>MNINEPSGEAANIISQAADSHAMKYYNAADWQAEDNALPSLAELRDLVINQQKSVLFDFSQNSDADGQAEMQAQFRKTYGVGFANQFIFITEHKGELLFTPFEHSEEVDPKLLEAPLTTRSGLKSTAPTNSETSTLPHVAFYISVNRPISDEECTFDNSWLWKDEKGSRPFCKDANISLIYRVNLERSLQYGIVGSATPNAKIVRISLDDDSSGAGIHLNDQLSYRRFGASYTTLDAYFREWSTDAIAQDYRFVFKTSNNKAEILETFPIDNLNVKYEKRKQSGFELGVTGGAEVSEDGPKAKLEARASITQSRWLTYNTQDYRVERNAKNAQTVSFTWNRQEYATAESLLNRSTDALWVDTYPVDVNRISPLSYASFVPKMDVIYKASDTETGSTDFIIDSSVNIRPIYNGAYKHYYVVGAHQSYHGFENSPRRRITKSASFTVDWDHPVFTGGRPVNLQLASFNNRCVQVDAQSRLTANTCDDQQSAQSFIYDQLGRYVSASNTELCLDGAALDVLQTCNQNLTQRWEWRKNTDELTNVYSGESLGHDKQTGELGLYASSNDAVSLRTITAYTNVFNVQKSSPILGYTQGKMNQQSVGQNYRLYVREGSAIDALGTASDLLVGGNGGSLTSVDLSGVKSITATSGDFQYGGQQLVALTFTYQDGRQQMVGSKAHVTNAHEDRFDLPDAAKITQLNIWADDWLVKGVQFDLNLEHHHHHH[7x]

Vibrio α-hemolysins (αHLs) are β-pore-forming toxins secreted by Vibrio pathogens, crucial for the facilitation of bacterial infections through host cell lysis. These toxins are produced as inactive precursors, requiring proteolytic maturation and membrane association for activation within host tissues. Here, we investigate Vibrio campbellii αHL (VcαHL), and establish that its hemolytic activity is significantly stimulated by calcium ions, with an EC50 that aligns with physiological calcium concentrations. Using X-ray crystallography and cryo-electron microscopy, we decipher both the immature and assembled structures of VcαHL and elucidate the conformational changes corresponding to toxin assembly.

The VcαHL was assembled on liposomal membranes and solubilized using styrene-maleic acid (SMA), yielding SMA lipid particles (SMALPs) containing assembled VcαHL. Cryo-micrographs of VcαHL in SMALPs were acquired and analyzed for single-particle 3D reconstitution, resulting in a density map of 2.06 Å resolution. The map revealed a heptameric complex exhibiting C7 symmetry, featuring a β-barrel transmembrane pore channel. In contrast, the β-prism lectin domain was not visualized in the map due to its flexible position in the complex, as indicated by the fuzzy cloud observed in 2D classification images. When compared to pro-VcαHL, the protomer of assembled VcαHL displays several conformational changes post pore formation, in addition to the substantial relocation of pre-stem loops. These include a slight clockwise rotation of the β-trefoil lectin domain when observed from the extracellular view and a minor displacement of the cradle loop, which seems to facilitate interaction with the adjacent protomer and release of the pre-stem loop. We thus attributed this extra-density to a calcium ion, coordinated with four water molecules, in line with the size of the density and the observed bond distance of 2.3–2.5 Å, typical features of a hydrated calcium ion. The hydrated calcium ions bind with H137 and E185, orienting the H137 to form a hydrogen bond with G194 from the cradle loop of an adjacent subunit. In addition, E185 in pro-VcαHL forms two hydrogen bonds with Q311 to maintain the association of the pre-stem loop with the cytolysin domain. These hydrogen bonds are replaced by coordination bonds with Ca2+ in assembled VcαHL, potentially facilitating the detachment of the pre-stem loop and triggering subsequent pore formation processes. In addition, the cryo-EM map of the assembled VcαHL uncovers a distinctive feature within the pore channel—an unassigned extra density located between the side chains of R279 and W314.>TDTIYHAKDAVQTTKPSERKPRLVVFVVGETARADHVQFNGYGRETFPQLAKVDGLANFSQVTSCGTSTAYSVPCMFSYLGQDDYDVDTAKYQENVLDTLDRLGVGILWRDNNSDSKGVMDKLPATQYFDYKSATNNTICNTNPYNECRDVGMLVGLDDYVSANNGK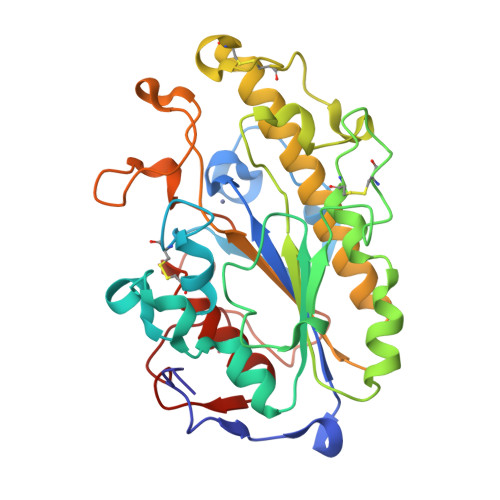DMLIMLHQMGNHGPAYFKRYDEQFAKFTPVCEGNELAKCEHQSLINAYDNALLATDDFIAKSIDWLKTHEANYDVAMLYVSDHGESLGENGVYLHGMPNAFAPKEQRAVPAFFWSNNTTFKPTASDTVLTHDAITPTLLKLFDVTAGKVKDRAAFIQ[2x]>GHMSPNYDKWEMERTDITMKHKLGGGQYGEVYEGVWKKYSLTVAVKTLKEDTMEVEEFLKEAAVMKEIKHPNLVQLLGVCTREPPFYIITEFMTYGNLLDYLRECNRQEVNAVVLLYMATQISSAMEYLEKKNFIHRDLAARNCLVGENHLVKVADFGLSRLMTGDTYTAHAGAKFPIKWTAPESLAYNKFSIKSDVWAFGVLLWEIATYGMSPYPGIDLSQVYELLEKDYRMERPEGCPE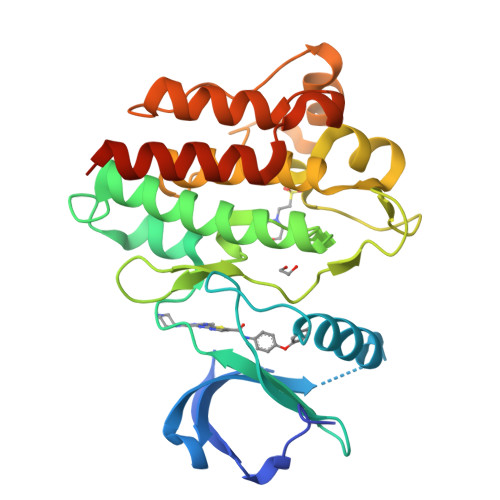KVYELMRACWQWNPSDRPSFAEIHQAFETMFQESSISDEVEKELGK[2x]>[2x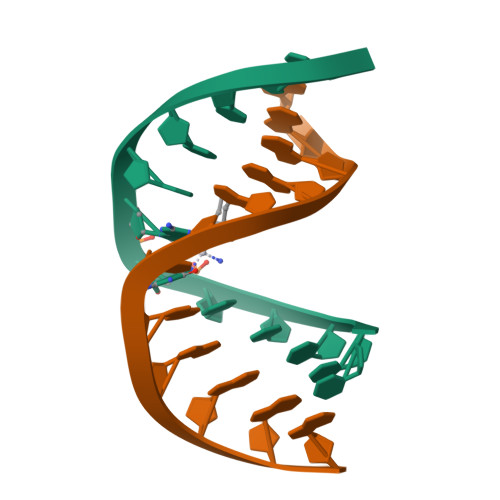]CCTCTGGTCTCC;>GGAGACCAGAGG[2x]>GSSGSSGHSVRVLQ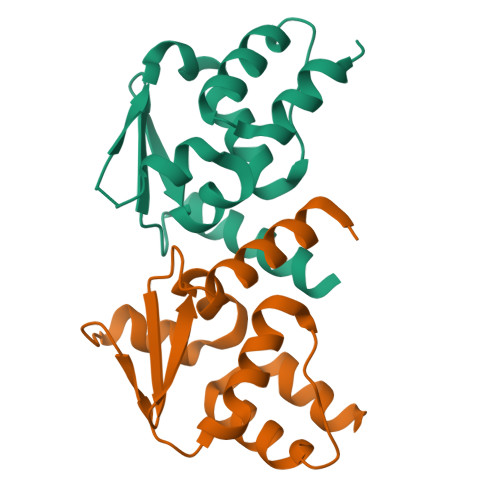ELNKQREKGQYCDATLDVGGLVFKAHWSVLACCSHFFQRIYGDGTGGSVVLPAGFAEIFGLLLDFFYTGHLALTSGNRDQVLLAAKELRVPEAVELCQSFQPQTSVGQAQSGLGQSGPSSG[2x]>[2x]MSSAAVAMLADPTVQIALACLVVSLFVVLQSVKKSKDEQTVYPVIAGMAIGNPQYRCTQNEALAVASKCPGLESIKPVLERIYGNSRIGSRYFAVPDFTPGRAAKGDPLFYPADGSYQVPVDVRLDKFKEKAVPLVSDVARRAIKEAGLNVEDISKLVVVSSTGFLGPGLDCELIKNLGLTRSVDRTLIGFMGCAAAMNGFRNANDYVTANPGKYALMICVELSSVHTTFDDNINDAILHA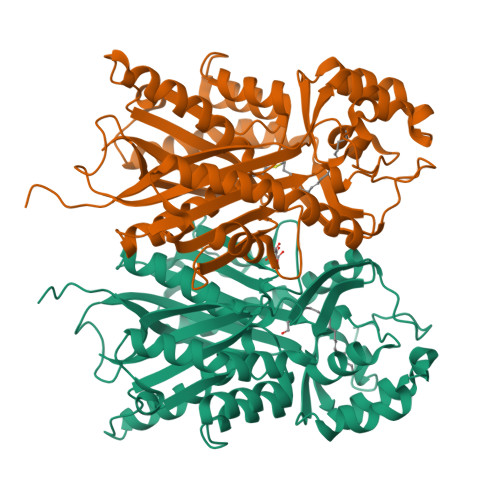IFADGCAAAVLKGARKSECPKGTLAIVDNHAWLMEGTEDGITLAIKPNGITCTLSKFLPQYIAKNIAFFADGFLKKHKLGRDDVDFWCVHPGGRRIIEEAQNGLGLSEEQTADSWAVLGEYGNMLSPSVMFVLSRVFKRHNAALAQGKPGYQTGMAFSFSPGVGAEGILLRQI>MAEKRTGLAEDGAKSVYERLKNDRAPYETRAQNCAQYTIPSLFPKDSDNASTDYQTPWQAVGARGLNNLASKLMLALFPMQTWMRLTISEYEAKQLLSDPDGLAKVDEGLSMVERIIMNYIESNSYRVTLFEALKQLVVAGNVLLYLPEPEGSNYNPMKLYRLSSYVVQRDAFGNVLQMVTRDQIAFGALPEDIRKAVEGQGGEKKADETIDVYTHIYLDEDSGEYLRYEEVEGMEVQGSDGTYPKEACPYIPIRMVRLDGESYGRSYIEEYLGDLRSLENLQEAIVKMSMISSKVIGLVNPAGITQPRRLTKAQTGDFVTGRPEDISFLQLEKQADFTVAKAVSDAIEARLSFAFMLNSAVQRTGERVTAEEIRYVASELEDTLGGVYSILSQELQLPLVRVLLKQLQATQQIPELPKEAVEPTISTGLEAIGRGQDLDKLERCVTAWAALAPMRDDPDINLAMIKLRIANAIGIDTSGILLTEEQKQQKMAQQSMQMGMDNGAAALAQGMAAQATASPEAM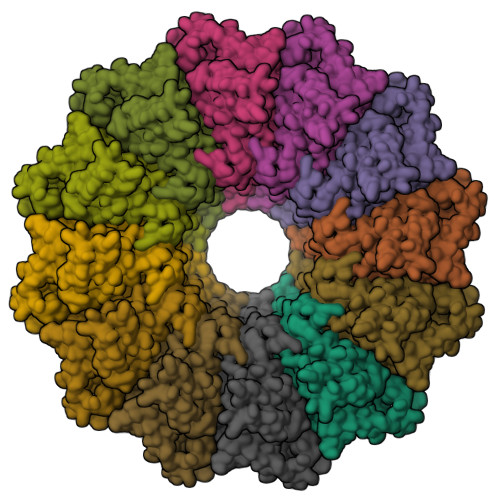AAAADSVGLQPGIAAALEHHHHHH[12x]1-phenyl-1H-imidazole | C9 H8 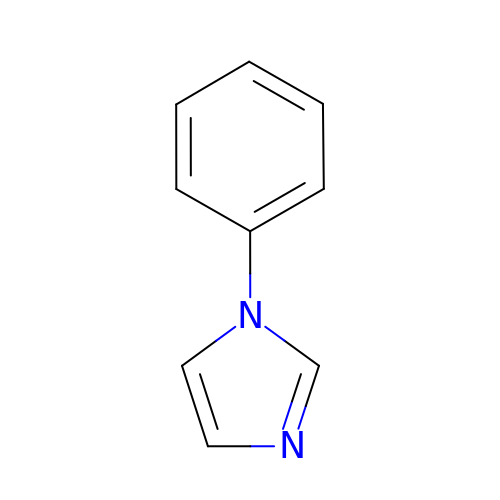N2 | SEULWJSKCVACTH-UHFFFAOYSA-N>[13x]MTNLQDQTQQIVPFIRSLLMPTTGPASIPDDTLEKHT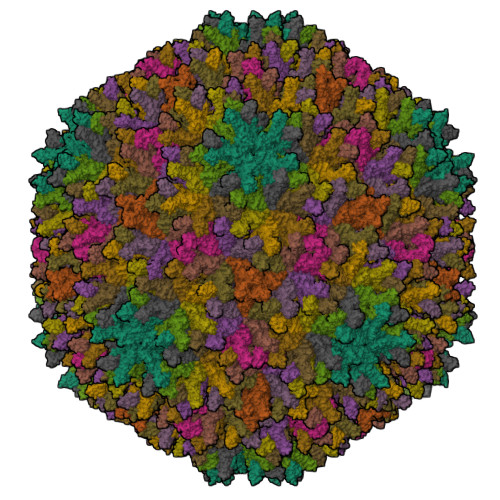LRSETSTYNLTVGDTGSGLIVFFPGFPGSIVGAHYTLQSNGNYKFDQMLLTAQNLPASYNYCRLVSRSLTVRSSTLPGGVYALNGTINAVTFQGSLSELTDVSYNGLMSATANINDKIGNVLVGEGVTVLSLPTSYDLGYVRLGDPIPAIGLDPKMVATCDSSDRPRVYTITAADDYQFSSQYQAGGVTITLFSANIDAITSLSIGGELVFQTSVQGLILGATIYLIGFDGTAVITRAVAADNGLTAGTDNLMPFNIVIPTSEITQPITSIKLEIVTSKSGGQAGDQMSWSASGSLAVTIHGGNYPGALRPVTLVAYERVATGSVVTVAGVSNFELIPNPELAKNLVTEYGRFDPGAMNYTKLILSERDRLGIKTVWPTREYTDFREYFMEVADLNSPLKIAGA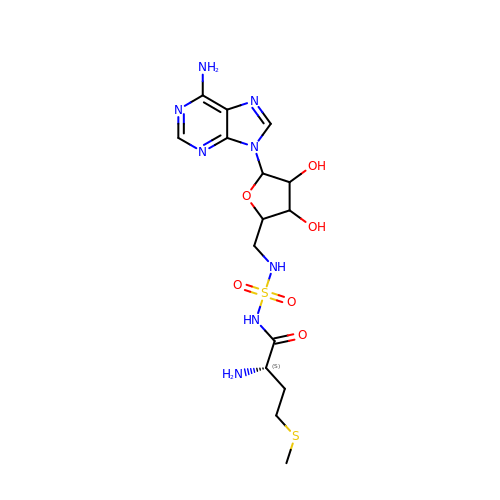N-[METHIONYL]-N'-[ADENOSYL]-DIAMINOSULFONE | C15 H24 N8 O6 S2 | DAUQVCLMADDCHF-QWRDWHBNSA-N>[2x]GSHMKISEFLHLALPEEQWLPTISGVLRQFAEEECYVYERPPCWYLGKGCQARLHINADGTQATFIDDAGEQKWAVDSIADCARRFM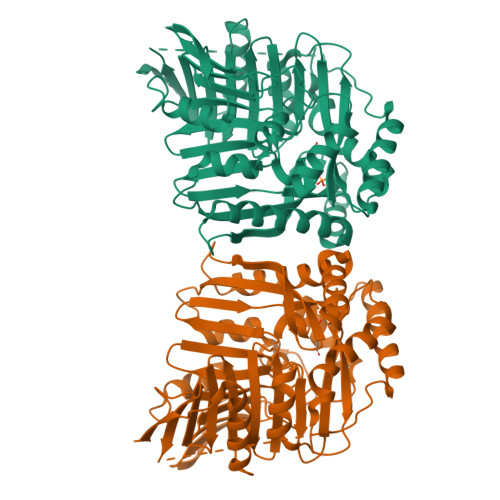AHPQVKGRRVYGQVGFNFAAHARGIAFNAGEWPLLTLTVPREELIFEKGNVTVYADSADGCRRLCEWVKEASTTTQNAPLAVDTALNGEAYKQQVARAVAEIRRGEYVKVIVSRAIPLPSRIDMPATLLYGRQANTPVRSFMFRQEGREALGFSPELVMSVTGNKVVTEPLAGTRDRMGNPEHNKAKEAELLHDSKEVLEHILSVKEAIAELEAVCLPGSVVVEDLMSVRQRGSVQHLGSGVSGQLAENKDAWDAFTVLFPSITASGIPKNAALNAIMQIEKTPRELYSGAILLLDDTRFDAALVLRSVFQDSQRCWIQAGAGIIAQSTPERELTETREKLASIAPYLMV> MSYASRTLGPMQTSSDRHEYPAHWEADVVLRDGGTARVRPITVDDAERLVSFYEQVSDESKYYRFFAPYPRLSAKDVHRFTH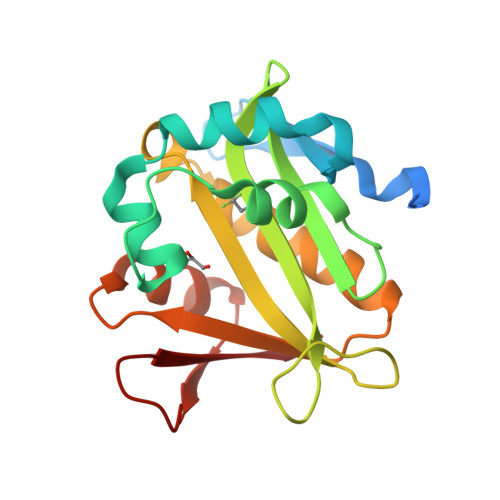HDFVDRVGLAATIGGEFIATVRYDRIGAGGTPATAPADEAEVAFLVQDAHQGRGVASALLEHIAAVARERGIRRFAAEVLPANNKMIKVFMDAGYTQKRSFEDGVVRLEFDL> GSDVVDP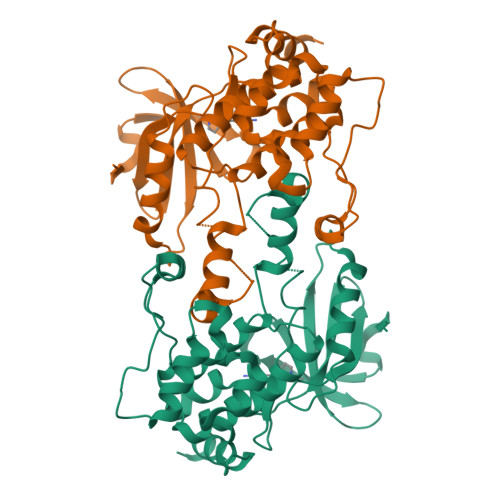DIFNRDPRDHYDLLQRLGGGTYGEVFKARDKVSGDLVALKMVKMEPDDDVSTLQKEILILKTCRHANIVAYHGSYLWLQKLWICMEFCGAGSLQDIYQVTGSLSELQISYVCREVLQGLAYLHSQKKIHRDIKGANILINDAGEVRLADFGISAQIGATLARRLAFIGTPYWMAPEVAAVALKGGYNELCDIWSLGITAIELAELQPPLFDVHPLRVLFLMTKSGYQPPRLKEKGKWSAAFHNFIKVTLTKSPKKRPSATKMLSHQLVSQPGLNRGLILDLLDKLKNGNS3-methyl-1-(2-methylpropyl)butyl 4-O-beta-L-gulopyranosyl-beta-D-glucopyranoside | C21 H40 O11 | 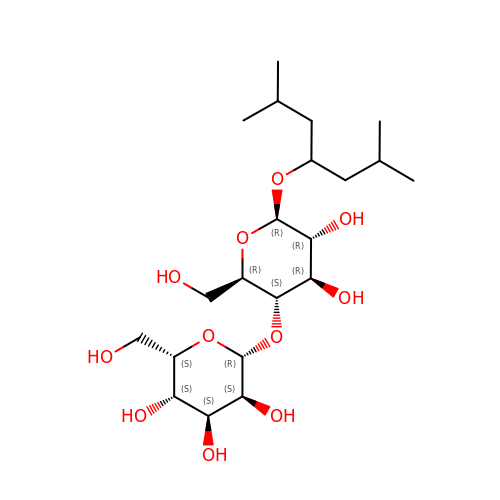RCXNRCWFTSDLDY-RDEKNSNJSA-N undecyl dihydrogen phosphate | C11 H25 O4 P | 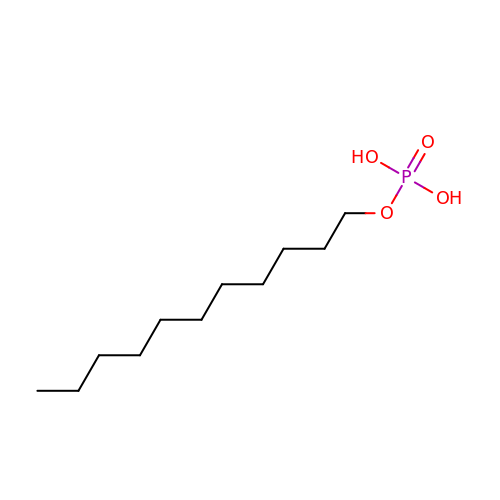VAIOGRPEROWKJX-UHFFFAOYSA-N>[2x]MSLNGSSIIEFEDMTWSQQVEDSKKPVVVMFYSPACPYCKAMEPYFEEYAKEYGSSAVFGRINIATNPWTAEKYGVQGT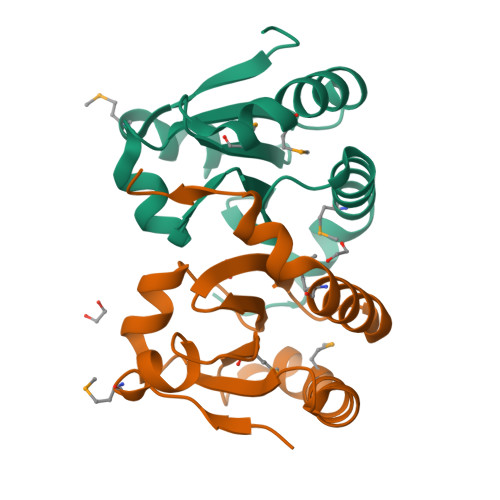PTFKFFCHGRPVWEQVGQIYPSILKNAVRDMLQHGEECIRKSTPVGQDITGYVEGHHHHHH>ARSEKRVPMTRLRKRVAERLLEAKNSTAMLTTFNEVNMKPIMDLRKQYGEAFEKRHGIRLGFMSFYVKAVVEALKRYPEVNASIDGDDVVYHNYFDVSMAVSTPRGLVTPVLRDVDTLGMADIE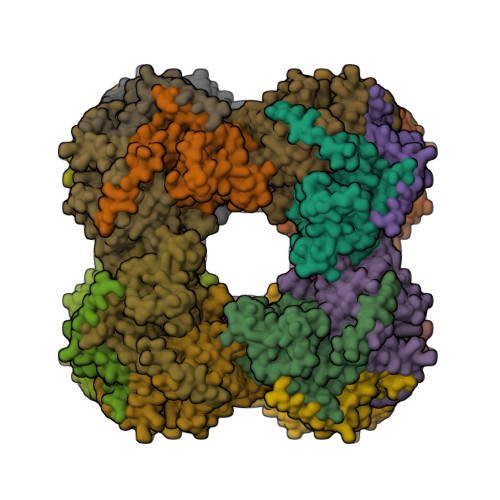KKIKELAVKGRDGKLTVEDLTGGNFTITNGGVFGSLMSTPIINPPQSAILGMHAIKDRPMAVNGQVEILPMMYLALSYDHRLIDGRESVGFLVTIKELLEDPTRLLLDV[24x]>MVDNSRTRPRVGHIQFLACLPLYWGLARTGTLLDFELTKDTPEKLSEQLVRGDLDIGPVTLVEFLKNADDLVAFPDIAVGCDGPVMSC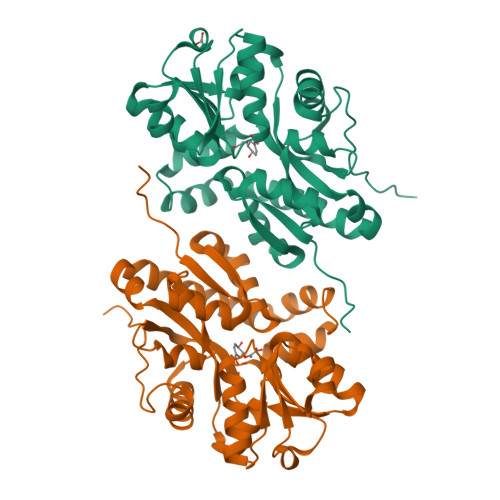VIVSQVPLDRLDGARVALGSTSRTSVRLAQLLLSERFGVQPDYYTCPPDLSLMMQEADAAVLIGDAALRANMIDGPRYGLDVHDLGALWKEWTGLPFVFAVWAARRDYAEREPVITRKVHEAFLASRNLSLEEVEKVAEQAARWEAFDEDTLAKYFTTLDFRFGAPQLEAVTEFARRVGPTTGFPADVKVELLKPLEHHHHHH[2x]> MKKLIPILEKIPEVELPVKEITFKEKLKWTGIVLVLYFIMGCIDVYTAGAQIPAIFGGTLITLGIGPIVTAGIIMQLLVGSGIIQMDLSIPENRALFQGCQKLLSIIMCFVEAVLFVGAGAFGILTPLLAFLVIIQIAFGSIILIYLDEIVSKYGIGSGIGLFIAAGVSQTIFVGALGPEGYLWKFLNSLIQGVPNIEYIAPIIGTIIVFLMVVYAECMRVEIPLAHGRIKGAVGKYPIKFVYVSNIPVILAAALFANIQLWGLALYRMGIPILGHYEGGRAVDGIAYYLSTPYGLSSVISDPIHAIVYMIAMIITCVMFGIFWVETTGLDPKSMAKRIGSLGMAIKGFRKSEKAIEHRLKRYIPPLTVMSSAFVGFLA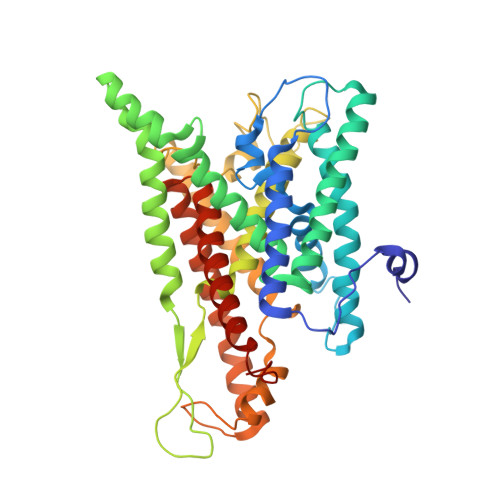TIANFIGALGGGTGVLLTVSIVYRMYEQLLREKVSELHPAIAKLLNK> AEEAFDLWNECAKACVLDLKDGVRSSRMSVDPAIADTNGQGVLHYSMVLEGGNDALKLAIDNALSITSDGLTIRLEGGVEPNKPVRYSYTRQARGSWSLNWLVPIGHEKPSNIKVFIHELNAGNQLSHMSPIYTIEMGDELLAKLARDATFFVRAHESNEMQPTLAISHAGVSVVMAQAQPRREKRWSEWASGKVLCLLDQLDGVYNYLAQQRCNLDDTWEGKIYRVLAGNPAKHDLDIKPTVISHRLHFPEGGSLAALTAHQACHLPLETFTRHRQPRGAEQLEQCGYPVQRLVALYLAARLSWNQVDQVIRNALASPGSGGDLGEAIREQPEQARLALTLAAAESERFVRQGTGNDEAGAANADVVSLTCPVAAGECAGPADSGDALLERNYPTGAEFLGDGGDVSFSTRGTQNWTVERLLQAHRQLEERGYVFVGYHGTFLEAAQSIVFGGVRARSQDLDAIWRGFYIAGDPALAYGYAQDQEPDARGRIRNGALLRVYVPRSSLPGFYRTSLTLAAPEAAGEVERLIGHPLPLRLDAITGPEEEGGRLETILGWPLAERTVVIPSAIPTDPRNVGGDLDPSSIPDKEQAISALPDYASQPGKPP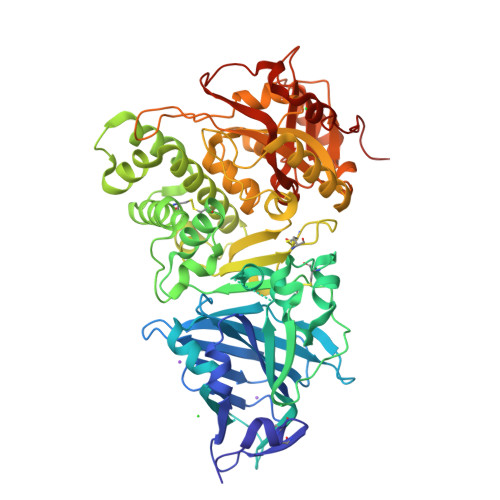REDLK> MKRVLIKPLEPLMFRSQGEFEPLITGSHTAAQSLIIPRPSTIAGMLGYILFNKSSGTGDWLSDLTNLLATIYGTFIETNGEYLFPLRMGNHLALVDQQHLINLPTLLEKEYERREKGIYELFYDKNKLFQIINHQDRIGISIDKSTRTVKEHYLYSARYLAFKKEVNYVIFIDNDAISDKINGKIVNFGGENRIAKLEVDDYKVDTSIEEEYYLALSPILIPDEALDNFLDNISDYVAMGKVDKISLGFDIANTKRKEMLTAILEGSIVKRSIIDFIKNEIKNDLRYRFSKYE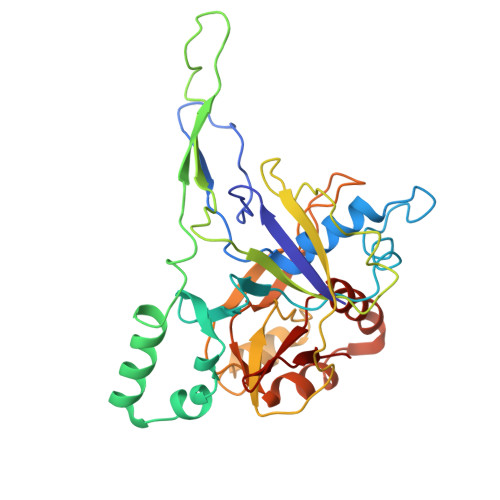KIGYNTLMSLCKLALRKILS>[24x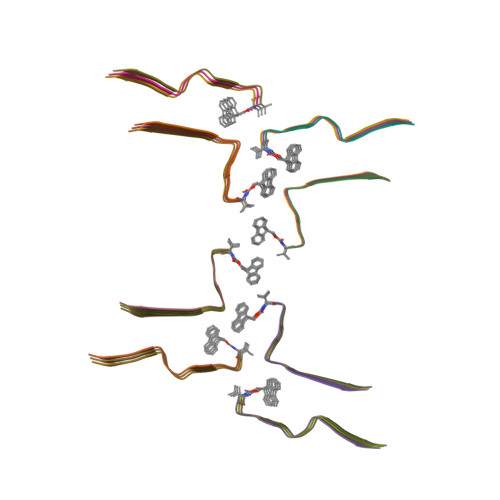]XVQSKIGSLDNITHX methyl (1R,3S)-1-methyl-3-[[3-[[3-methyl-4-[(4-pyridin-3-ylpyrimidin-2-yl)amino]phenyl]carbamoyl]phenyl]carbamoyl]-4-oxidanylidene-cyclohexane-1-carboxylate | C33 H32 N6 O5 | 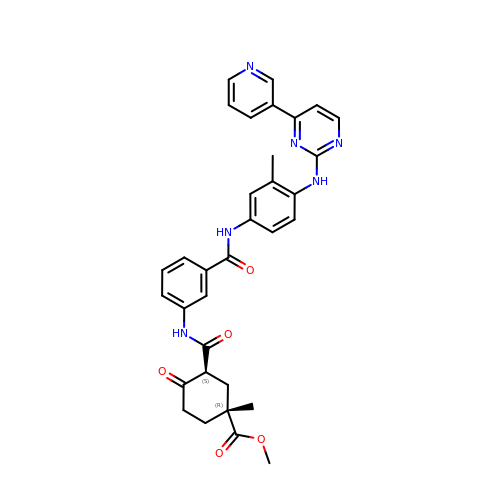LOKFZRXMKAWKTK-OGVWKLGRSA-N(2S)-2-{[(S)-(2-carboxyethyl)(hydroxy)phosphoryl]methyl}pentanedioic 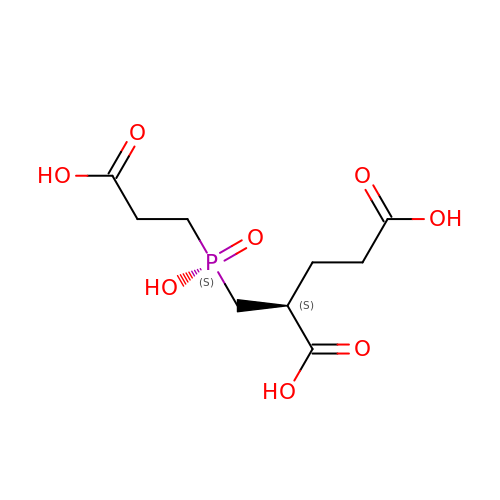acid | C9 H15 O8 P | GZNKYXXCKRYSFH-ZCFIWIBFSA-N> DRVELN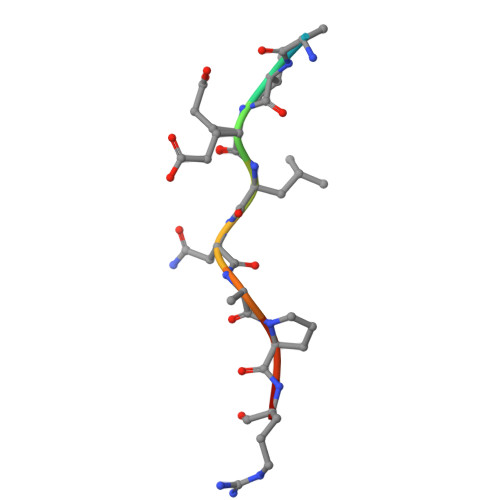APRQ> MKKILFDVDGVFLSEERCFDVSALTVYELLMDKCYLGLHSHIDWETLTDNDIQDIRNRIFQKDKILNKLKSLGLNSNWDMLFIVFSIHLIDILKKLSHDEIEAFMYQDEPVELKLQNISTNLADCFNLNEQLPLQFLDNVKVGKNNIYAALEEFATTELHVSDATLFSLKGALWTLAQEVYQEWYLGSKLYEDVEK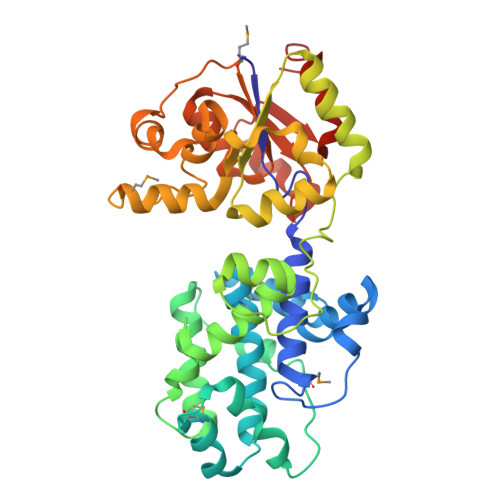KIARTTFKTGYIYQEIILRPVDEVKVLLNDLKGAGFELGIATGRPYTETVVPFENLGLLPYFEADFIATASDVLEAENMYPQARPLGKPNPFSYIAALYGNNRDKYESYINKQDNIVNKDDVFIVGDSLADLLSAQKIGATFIGTLTGLKGKDAAGELEAHHADYVINHLGELRGVLDNLLEHHHHHH> MYGSTTARNLPSGKKQRIADLLSQIIETLDLTKTQYANIESAYNGVGTFLSEGDDPLLQDAVIYPQGSVRLNTTVKPKNEEQYDIDLICYLPHATQADYTGVISAIRQRLESHKTYKTLLSELPRGFRINYAGDYHLDITPGRDHTGTAHPGQPLWVVDAQTAWKESNPSGYAEWFESSASVQPLRTILVMDSASRVGTEALLPLPDST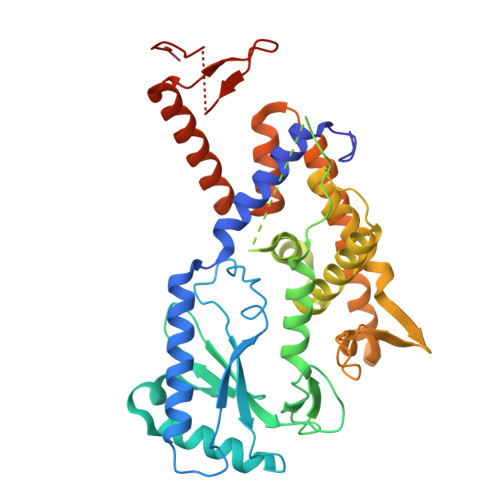DKKLLNHIVQILKRHRDEWAAEQDEVRQRCRPISVIITTLACHAYNHIIADRRAYDNDLDILLDVLELMPDFIVSTQGAIHVNNPHMPEENFAEKWNRSEQDEGPQRSEAFYQWHAAAQATFNTIAASVGEDNLFLSLEDSFGKTPVDVVRQRLMEHMQSAREQGSLHLDKKTGGLIATGLAGTAAQAGVPKNTFYGE> MSVGKPLPHDSARAHVTGQARYLDDLPCPANTLHLAFGLSTEASAAITGLDLEPVRESPGVIAVFTAADLPHDNDASPAPSPEPVLATGEVHFVGQPIFLVAATSHRAARIAARKARITYAPRPAILTLDQALAADSRFEGGPVIWARGDVETALAGAAHLAEGCFEIGGQEHFYLEGQAALALPAEGGVVIHCSSQHPSEIQHKVAHALGLAFHDVRVEMRRMGGGFGGKESQGNHLAIACAVAARATGRPCKMRYDRDDDMVITGKRHDFRIRYRIGADASGKLLGADFVHLARCGWSADLSLPVCDRAMLHADGSYFVPALRIESHRLRTNTQSNTAFRGFGGPQGALGMERAIEHLARGMGRDPAELRALNFYDPPERGGLSAPPSPPEPIATKKTQTTHYGQEVADCVLGELVTRLQKSANFTTRRAEIAAWNSTNRTLARGIALSPVKFGISFTLTHLNQAGALVQIYTDGSVALNHGGTEMGQGLHAKMVQVAAAVLGIDPVQVRITATDTSKVPNTSATAASSGADMNGMAVKDACETLRGRLAGFVAAREGCAARDVIFDAGQVQASGKSWRFAEIVAAAYMARISLSATGFYATPKLSWDRLRGQGRPFLYFAYGAAITEVVIDRLTGENRILRTDILHDAGASLNPALDIGQIEGAYVQGAGWLTTEELVWDHCGRLMTHAPSTYKIPAFSDRPRIFNVALWDQPNREETIFRSKAVGEPPFLLGISAFLALH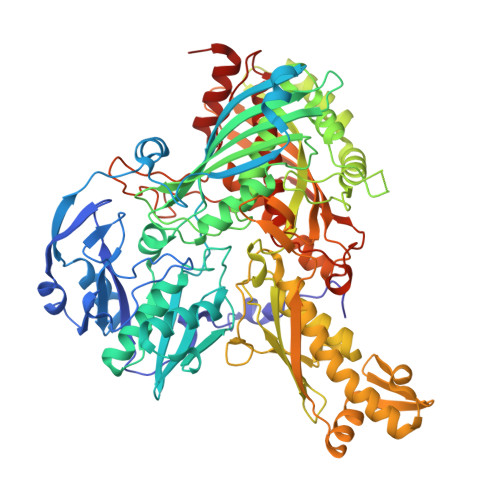DACAACGPHWPDLQAPATPEAVLAAVRRAEGRA>MRGSHHHHHHGIQMVSIAINGFGRIGRLVLRIALERKNIDVVAINDPFISVDYAAYMFKYDSTHGKYKGEVSHDGSNLIINGKKVAVFQEKDPATLPWGKLGVDIAVDSTGVFKELDSAQKHIDAGAKKVVITAPSKTAPMFVVGVNEDKYNGEKIVSNASCTTNCLAPIAKIINDEFGIEEGLMTTVHSITATQKTVDGPSHKDWRGGRTASGNIIPSSTGAAKAVGKVLPELQGKLTGMAFRVPTTDVSVVDLTVKLVKAATYDEIKAAVKKVSEGKLKDVVG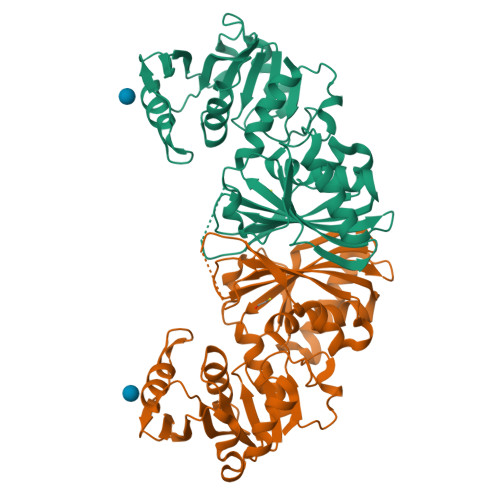YTEDAVVSSDFLGDTHSTIFDAAAGIQLSPKFVKLVAWYDNEYGYSTRVVDLVEHVA[2x]>MRGSHHHHHHGSMRKPIIGVMGPGEQATPTDLKNAYQLGQLIALEGWVLLTGGRNVGVMEHASQGAKKAEGLTIGILPSKNTHNVSDAVDIAIVTGLGNARNNINVLSSDVVIACGIGLGTLSEVALALKNQKPVILLNDDLLSQELFANLSNNQVWIASSPENCIELIKSIITVKLN[4x]

The green alga Chlamydomonas reinhardtii harbors a Moco carrier protein (MCP) that binds and protects Moco but is devoid of enzymatic function. Moco carrier proteins (MCPs) neither belong to the Moco-biosynthesis pathway nor qualify as Mo-enzymes as they are non-enzymatic proteins within molybdenum metabolism. In the present work, we identified and characterized the first confirmed Moco carrier protein originating from a prokaryotic organism, the cyanobacterium R. orientalis. We showed that RoMCP selectively binds Moco and discriminates it from its dinucleotide derivatives.

We chose the MCP homolog from the organism R. orientalis, a cyanobacterium belonging to the genus Rippkaea, a recently established phylogenetic lineage formerly assigned to the genus Cyanothece. This putative MCP, referred to in the following as RoMCP, consists of 163 amino acids corresponding to a molecular weight of 17.1 kDa and shares 52.5% sequence identity with CrMCP. A monomer of the RoMCP construct in the crystal structure comprises 178 amino acids, 15 of which correspond to affinity and cloning tags. The electron density allowed the modeling of all amino acids of RoMCP in an uninterrupted polypeptide chain. In contrast, most amino acids of the affinity and cloning tags show disorder. An RoMCP monomer contains five α-helices (h1, h2, h4, h5 and h6) and one mixed helix (h3) that begins in a 310 conformation and ends in an α conformation. The helices lie below (h1, h2 and h6) and above (h3, h4 and h5) a parallel β-sheet, resulting in a three-layered sandwich structure that resembles a Rossmann fold. In contrast to the canonical, six-stranded Rossmann fold, a seventh strand (denominated β4) expands the β-sheet of RoMCP, resulting in an arrangement with the order β4β3β2β1β5β6β7. A nonregular stretch of amino acids between β1 and h1 contains the Rossmann consensus sequence GxGxxA/G that is usually involved in nucleotide binding. However, CrMCP exhibits a tetrameric quaternary structure with 222 point-group symmetry generated from the content of the asymmetric unit by a twofold crystallographic rotation axis. This tetrameric assembly is identical to the content of the asymmetric unit in the RoMCP structure. PISA estimated the solvation free-energy gain upon the formation of dimer AB to be 90.0 kJ mol−1, which is significantly greater than that for the formation of dimer AC (55.6 kJ mol−1), indicating that the formation of the RoMCP tetramer follows the route via a dimer AB intermediate. We thus reason that the positively charged crevice and the chloride anions bound within it mark the putative Moco-binding site of RoMCP.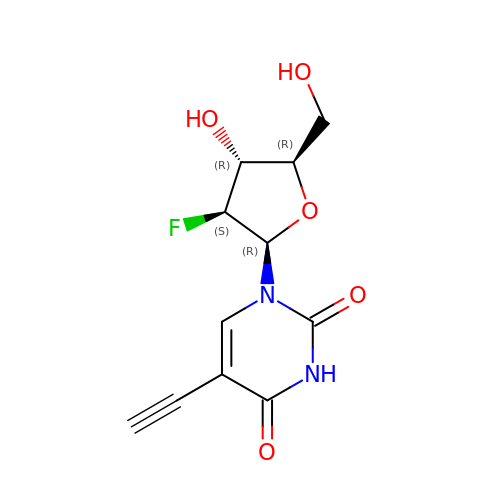1-(2-deoxy-2-fluoro-beta-D-arabinofuranosyl)-5-ethynylpyrimidine-2,4(1H,3H)-dione | C11 H11 F N2 O5 | YEEGMPUOCRQFRV-IBCQBUCCSA-N> DNVLLSGQTLHADHSLQAGAYTLTIQNKCNLVKYQNGRQIWASNTDRRGSGCRLTLLSDGNLVIYDH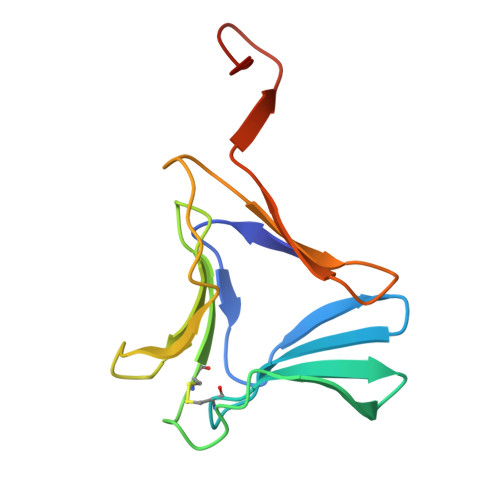NNNDVWGSACWGDNGKYALVLQKDGRFVIYGPVLWSLGPNGCRRVNG Bacterial hybrid malic enzymes (MaeB grouping, multidomain) catalyse the transformation of malate to pyruvate, and are a major contributor to cellular reducing power and carbon flux. Distinct from other malic enzyme subtypes, the hybrid enzymes are regulated by acetyl-CoA, a molecular indicator of the metabolic state of the cell. The larger ME isoforms (hybrid enzymes) are predicted to be a fusion of two unrelated enzymes; a catalytic N-terminal ME subunit and a C-terminal phosphotransacetylase (PTA) domain. The PTA domain is homologous to PTA enzymes (that interconvert acetyl-CoA and phosphate to CoA and acetyl phosphate), yet they appear to lack critical catalytic residues and thus acts as a sensor instead.

We were successful in obtaining the acetyl-CoA bound inhibited state (MaeBbound), diffracting to 2.72 Å resolution. Full-length MaeBbound retains the architectures observed for the isolated structures, placing the ME dimer twofold axis immediately below that of the PTA d2:d2 dimer axis. The folds are in excellent agreement with those observed in isolation (0.6 Å rmsd between ME domain structures, 1.2 Å between PTA domain structures). The resultant hexamer forms a disc measuring ~100 × 175 × 195 Å, with the ME domains twisted with respect to the triangular PTA edge. The individual ME and PTA domains are linked by two α-helices, the first, referred to here as L1, composed of a region unique to hybrid MEs (residues 422–437), and the second, L2, formed from the first α-helix of the PTA fold (residues 438–457). The relative orientation of the ME and PTA domains results in very few contacts between the two—L1 packs against the ME core via several conserved hydrophobic residues and L2 is ampipathic, with a hydrophobic N-terminus interacting with the PTA d1:d2 interface, and a polar C-terminus partly solvent-exposed. A key structural feature of the inhibited conformation of MaeB is the presence of a clash between the L2 helix and the ME domain surface, which results in the disordering of the ME hook subdomain. Disorder of the hook is apparent in all six chains of the hexamer, with small differences (chains A–D disordered from residues 371–383, residues 370–379 in chains E and F). Interestingly, residue F386 at the base of the hook is an equivalent position to human ME residue L507, which has been shown to be involved in the conversion to the closed catalytically active state. It is likely that our inhibited MaeBbound structure represents an inactive state by both disordering the local hook structure and limiting the dynamics of d1.

>MGSSHHHHHHSMDNKTETKIEPKTGTTNFDQEALLYHQQGKPGKIEVISSKPCATEKDLSLAYSPGVAAPCKAIAKDPAKVYDYTAKGNLVAVISNGTAVLGLGNIGPAAGKPVMEGKGILFKQFAGIDVFDIEVAATDVDVFCNAVRVLEPTFGGINLEDIKAPECFEIEERLKKEMNIPVFHDDQHGTAIVSGAALLNACSITNRKMETVRIVVNGAGASANSCAKIFIALGARRENIIMCDSQGVIYKGRTAGMNKYKEYFASETEARTLTEALRGADVFVGLSVAGALTPEMLKDMAKDPIIFAMANPEPEITPDKARAARPDAIIATGRSDYPNQVNNVLGFPSIFRGALDTRSTQINEEMKLAAVHALAKLAREDVPDKVSATYGGKSFKFGRDYLIPKPFDTRVLLWVAPEVAKAAMKSGVATRAIEDWDQYRESLEALQGPSKVFIRSAINRVHQNSAANGGELPRIVFPEGTSTKVLKALATLVEEKICQPILLGYPERVKEKIKALDIPLLNDVSIVHPSSHPKYFSFVEKLYSLRQRKGINLGEAERLMADPNYFAAMMVNQGEADGMVSGSSINYADAVRPILQTIGVYKEGIPAGLNFVLLEDKFLVLADTTVNLNPTAEQCAQIALQAAKIVEYFGIEPRVAMLSYSNFSGAEGTPRKMKKAAEIARSLRPDLMIEGDMQADTAVNPEIMERLFPFSGLKGGANVLVFPNLESSNIAYKLIQQIGKAEVIGPFLTGVRRSANVLQRTTTVDGIVNSVVFTALEAQYIKEVLKSRGKK[6x]>HHHHHHMSMKSQFERAKIEYGQWGIDVEEALERLKQVPISIHCFQGDDVGGFELSKGELSGGIDVTGDYPGKATTPEELRMDLEKALSLIPGKHRVNLHAIYAETDGKVVERDQLEPRHFEKWVRWAKRHGLGLDFNPTLFSHEKAKDGLTLAHPDQAIRQFWIDHCIASRKIGEYFGKELETPCLTNIWIPDGYKDTPSDRLTPRKRLKESLDQIFAAEINEAYNLDAVESKLFGIGSESYVVGSHEFYLSYALKNDKLCLLDTGHYHPTETVSNKISAMLLFHDKLALHV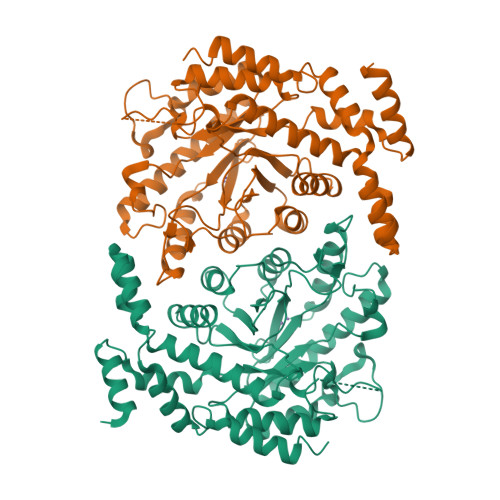SRPVRWDSDHVVTFDDELREIALEIVRNDALDRVLIGLDFFDASINRIAAWTIGTRNVIKALLFAMLIPHKQLKEWQETGDYTRRLAVLEEFKTYPLGAIWNEYCERMNVPIKEEWLKEIAIYEKEVLLQRH[4x]>RICFNHQSSQP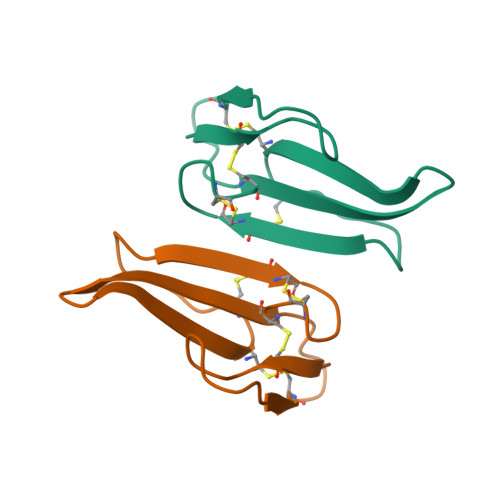QTTKTCSPGESSCYNKQWSDFRGTIIERGCGCPTVKPGIKLSCCESEVCNN[2x]> 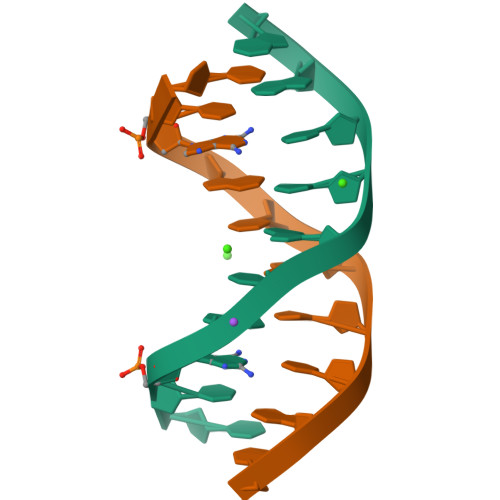CCAGTACTGG> MANVWGVRLADSLSSPTIETRTRQYTLHDLCSDLDANPGREPWKPLRNQRTNNIVAVQLFRPLQGLVLDTQLYGFPGAFDDWERFMREKLRVLKYEVLRIYPISNYSNEHVNVFVANALVGAFLSNQAFYDLLPLLIINDTMIGDLLGTGASLSQFFQSHGDVLEVAAGRKYLQMENYSNDDDDPPLFAKDLSDYAKAFYSDTYEVLDRFFWTHDSSAGVLVHYDKPTNGHHYLLGTLTQMVSAPPYIINATDAMLLESCLEQFSANVRARPAQPVTRLDQCYHLRWGAQYVGEDSLTYRLGVLSLLATNGYQLARPIPRQLTNRWLSSFVSQIMSDGVNETPLWPQERYVQIAYDSPSVVDGATQYGYVRKNQLRLGMRISALQSLSDTPSPVQWLPQYTIDQAAMDEGDLMVSRLTQLPLRPDYGNIWVGDALSYYVDYNRSHRVVLSSELPQLPDTYFDGDEQYGRSLFSLARKIGDRSLVKDTAVLKHAYQAIDPNTGKEYLRSRQSVAYFGASAGHSGADQPLVIEPWIQGKISGVPPPSSVRQFGYDVARGAIVDLARPFPSGDYQFVYSDVDQVVDGHDDLSISSGLVESLLSSCMHATAPGGSFVVKINFPTRPVWHYIEQKILPNITSYMLIKPFVTNNVELFFVAFGVHQHSSLTWTSGVYFFLVDHFYRYETLSTISRQLPSFGYVDDGSSVTGIETISIENPGFSNMTQAARIGISGLCANVGNARKSIAIYESHGARVLTITSRRSPASARRKSRLRYLPLIDPRSLEVQARTILPADPVLFENVSGASPHVCLTMMYNFEVSSAVYDGDVVLDLGTGPEAKILELIPATSPVTCVDIRPTAQPSGCWNVRTTFLELDYLSDGWITGVRGDIVTCMLSLGAAAAGKSMTFDAAFQQLIKVLSKSTANVVLVQVNCPTDVVRSIKGYLEIDSTNKRYRFPKFGRDEPYSDMDALEKICRTAWPNCSITWVPLSYDLRWTRLALLESTTLSSASIRIAELMYKYMPIMRIDIHGLPMEKRGNFIVGQNCSLVIPGFNAQDVFNCYFNSALAFSTEDVNAAMIPQVSAQFDATKGEWTLDMVFSDAGIYTMQALVGSNANPVSLGSFVVDSPDVDITDAWPAQLDFTIAGTDVDITVNPYYRLMTFVRIDGQWQIANPDKFQFFSSASGTLVMNVKLDIADKY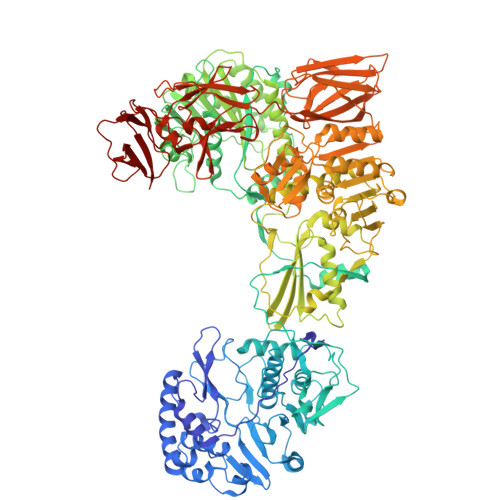LLYYIRDVQSRDVGFYIQHPLQLLNTITLPTNEDLFLSAPDMREWAVKESGNTICILNSQGFVLPQDWDVLTDTISWSPSIPTYIVPPGDYTLTPL>[2x]GSKEGEYIKL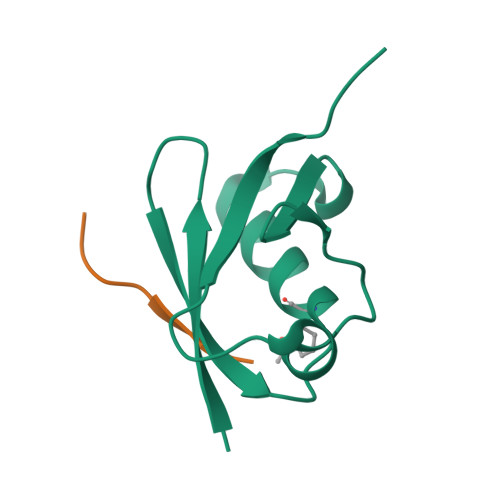KVIGQDSSEIHFKVKMTTHLKKLKESYAQRQGVPMNSLRFLFEGQRIADNHTPKELGMEEEDVIEVYQEQTGG;>[2x]GSGEAEERIIVLSDSDY>GSGREEDPHEGKIWFHGKISKQEAYNLLMTVGQVSSFLVRPSDNTPGDYSLYFRTNENIQRFKISPTP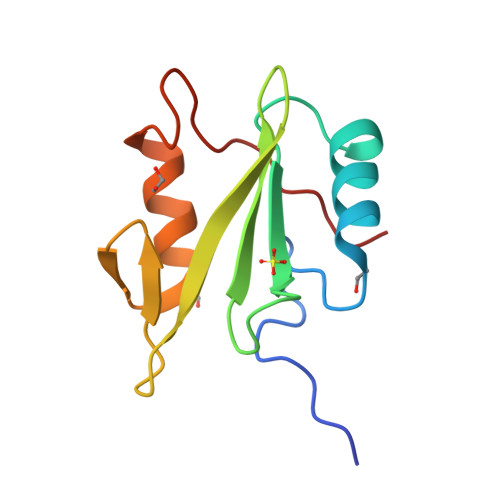NNQFMMGGRYYNSIGDIIDHYRKEQIVEGYYLKEPVPMQ[2x]>[8x]MAELACFCYP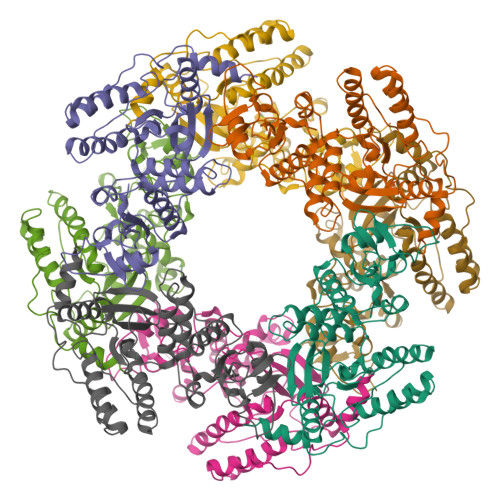HLENDSYKFIPFNNLAIKAMLTAKVDKKDMDKFYDSIIYGIAPPPQFKKRYNTNDNSRGMNFETIMFTKVAMLICEALNSLKVTQANVSNVLSRVVSIRHLENLVIRKENPQDILFHSKDLLLKSTLIAIGQSKEIETTITAEGGEIVFQNAAFTMWKLTYLEHQLMPILDQNFIEYKVTLNEDKPISDVHVKELVAELRWQYNKFAVITHGKGHYRIVKYSSVANHADRVYATFKSNVKTGVNNDFNLLDQRIIWQNWYAFTSSMKQGNTLDVCKRLLFQKMKPEKNPFKGLSTDRKMDEVS>HHHHHHSSGLVPRGSHMLKLLEPFDLNGLELANRMVMAPLTRNRAGPRFVPTKMNALYYAQRSGLGLIITEATQISQQGMGYPDTPGIYTDEQVDGWRMVTEAVHRREGCIFLQLWHVGRVSHSSFQPNGQLPVAPSAIAPEGEVMTYDGIKPFETPRALETEEVAHIVEDYRKAAINAKRAGFDGIEIHSANGYLLHEFLEDGTNKRTDRYGGSIENRARIVFEVLDAVCKVYPSRRVGIRLSPDTEFMSMSDSDRPALYSYLVQELSRRELAYLHLIEPRIKGNVDVEKESSLNVEFFRPLYKGVLITAGGYQKETGEERLQKQHADLVAYGRWVIANPDLPSRFEQNAPLNPYDRATFYGGNEKGYTDYPFLDPRDSQEALKEAEAAERKWR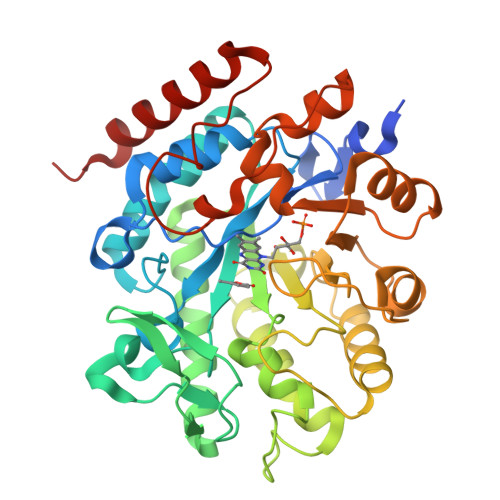RL[2x]VITAMIN E | C29 H50 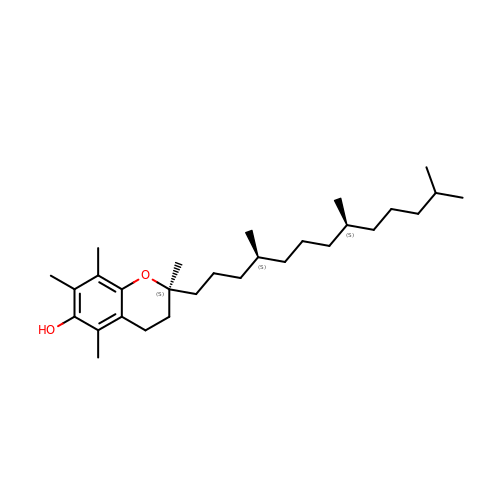O2 | GVJHHUAWPYXKBD-SYZUXVNWSA-N>[2x]NCTLSKGFTTVDIPMTIGTIVVRPTDPIGTVLQKNTFTI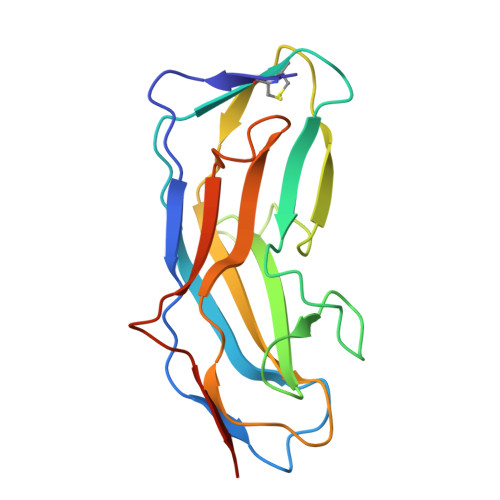SPNNSTATCNRASDQITAALPLNYPVSSIGNNVYATNIPGIGIRLYREAFDSTDFSGYYPYKRSLTPNTTYTLSPGYFVMEVIKTAATTGSGALVAGRYSTYYVTGQQNRPFLTTTVLSSSPILIASSSHHHHHH>[3x]GSHMFTGLNTP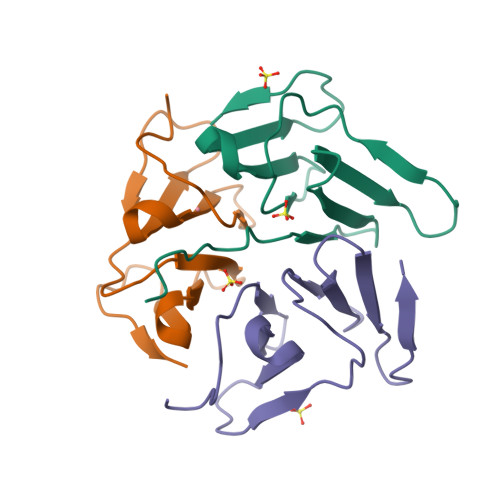HGVAVDSAGTVYVTDHGNNRVVKLAAGSNTQTVLPFTGLNTPSGVAVDSAGTVYVTDHGNNRVVKLAAGSNTQTVL The DNA damage response protein 53BP1 (p53-binding protein 1) influences the cell cycle dependency of DNA double-strand break (DSB) repair pathway selection. The localization of 53BP1 to chromatin also requires that it binds histone H4 di-methylated at K20 (H4K20me2) via a tandem Tudor domain (53BP1TT), while BRCA1-BARD1 recruitment requires unmethylated H4K20 recognized by an Ankyrin repeat domain in BARD1. We show that a series of water-soluble small molecules targeting the methyl-lysine binding cavity in 53BP1TT function by stabilizing a previously unknown lowly populated autoinhibited homodimeric state of 53BP1TT in which the histone binding surface of H4K20me2 is buried within the protomeric interface. Our work therefore identifies an auto-associated form of 53BP1—autoinhibited for chromatin binding—that can be stabilized by small molecule ligands encapsulated between two 53BP1 protomers.

Our structural characterization of 53BP1TT in complex with the related compounds UNC2991 (Kd = 3.9 ± 0.4 μM), UNC3351 (Kd = 6.8 ± 0.4 μM) and UNC3474 (Kd = 1.0 ± 0.3 μM) revealed a similar three-dimensional (3D) arrangement wherein each ligand not only blocked the methyl-lysine binding site but was encapsulated in a cavity generated by two 53BP1TT molecules. This consistent burial of the histone binding surface of 53BP1TT by dimerization was unexpected. Since the homodimerization interface in the crystal structures buries the histone binding surface of 53BP1TT, such a conformation would be autoinhibitory for chromatin binding. Several of the 53BP1TT residues that are close to the small molecule binding site had two different NMR signals. This is consistent with loss of symmetry observed in our crystal structures, allowing interactions by each of the two 53BP1TT protomers with a different “side” of the bound small molecule. Taken together, our data demonstrate that like in the crystal structures, the small molecules are buried at the interface of a 53BP1TT homodimer in solution.

>[2x]GHMNSFVGLRVVAKWSSNGYFYSGKITRDVGAGKYKLLFDDGYECDVLGKDILLCDPIPLDTEVTALSEDEYFSAGVVKGHRKESGELYYSIEKEGQRKWYKRMAVILSLEQGNRLREQYGLG> ADTVTLPFANGERPLVMYPGKRPLIGLTARPPQLETPFSVFDEGLITPNDAFFVMYHLAGIPLEIDPDAFRLEIKGKVGTPLSLSLQDLKNDFPASEVVAVNQCSGNSRGFVEPRVGGGQLANGAMGNARWRGVPLKAVLEKAGVQAGAKQ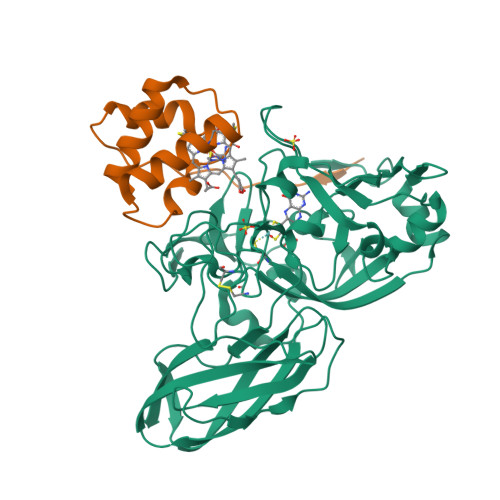VTFGGLDGPVIPETPDFVKALSIDHATDGEVMLAYSMNGADLPWLNGYPLRLVVPGYYGTYWVKHLNEITVIDKEFDGFWMKTAYRIPDNACACTEPGKAPTATIPINRFDVRSFITNVENGASVKAGEVPLRGIAFDGGYGITQVSVSADAGKSWTNATLDPGLGKYSFRGWKAVLPLTKGDHVLMCRATNARGETQPMQATWNPAGYMRNVVEATRVIAA;> APLTYELPDETAQLKPAPQPGFEAAQNNCAACHSVDYINTQPPGKGQAFWDAEVQKMIKVYHAPVDEADAKAIADYLAKTY> GAMWHTHSEREKRVSNAVEFLLDSRVRRTPTSSKVHFLKSK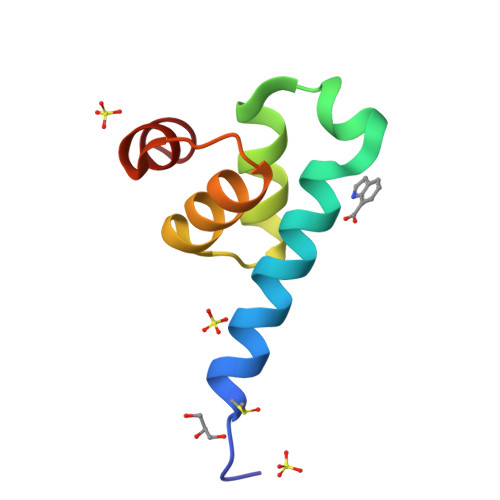GLSAEEICEAFTKVGQPKTLNEIKRILS>[2x]GPEFSMEDLIPLVNRLQDAFSAIGQNADLDLPQIAVVGGQSAGKSSVLENFVGRDFLPRGSGIVTRRPLVLQLVNATTEYAEFLHCKGKKFTDFEEVRLEIEAETDRVTGTNKGISPVPINLRVYSPHVLNLTLVDLPGMTKVPVGDQPPDIEFQIRDMLMQFVTKENCLILAVSPANSDLANSDALKVAKEVDPQGQRTIGVITKLDLMDEGTDARDVLENKLLP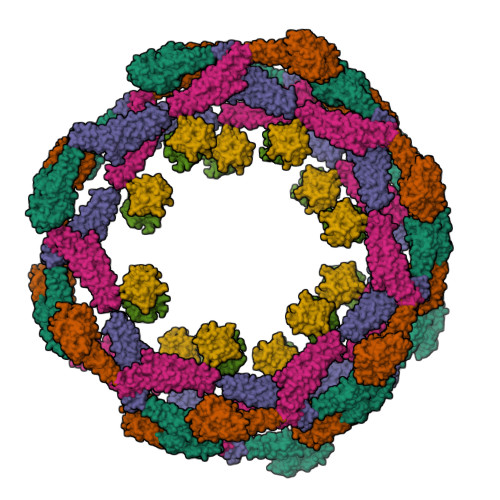LRRGYIGVVNRSQKDIDGKKDITAALAAERKFFLSHPSYRHLADRMGTPYLQKVLNQQLTNHIRDTLPGLRNKLQSQLLSIEKEVEEYKNFRPDKHGTDSRVDEMLRMYHALKEALSIIGNINTTTV;>[2x]MVVSEVDIAKADPAAASHPLLLNGDATVAQKNPGSVAENNLCSQYEEKVRPCIDLIDSLRALGVEQDLALPAIAVIGDQSSGKSSVLEALSGVALPRGSGIVTRCPLVLKLKKLVNEDKWRGKVSYQDYEIEISDASEVEKEINKAQNAIAGEGMGISHELITLEISSRDVPDLTLIDLPGITRVAVGNQPADIGYKIKTLIKKYIQRQETISLVVVPSNVDIATTEALSMAQEVDPEGDRTIGILTKPDLVDKGTEDKVVDVVRNLVFHLKKGYMIVKCRGQQEIQDQLSLSEALQREKIFFENHPYFRDLLEEGKATVPCLAEKLTSELITHICKSLPLLENQIKETHQRITEELQKYGVDIPEDENEKMFFLIDKVNAFNQDITALMQGEETVGEEDIRLFTRLRHEFHKWSTIIENNFQEGHKILSRKIQKFENQYRGRELPGFVNYRTFETIVKQQIKALEEPAVDMLHTVTDMVRLAFTDVSIKNFEEFFNLHRTAKSKIEDIRAEQEREGEKLIRLHFQMEQIVYCQDQVYRGALQKVREKELEEEKKKKSWDFGAFQSSSATDSSMEEIFQHLMAYHQEASKRISSHIPLIIQFFMLQTYGQQLQKAMLQLLQDKDTYSWLLKERSDTSDKRKFLKERLARLTQARRRLAQFPG;>[2x]ILVIRKGWLTINNIGIMKGGSKEYWFVLTAENLSWYKDDEEKEKKYMLSVDNLKLRDVEKGFMSSKHIFALFNTEQRNVYKDYRQLELACETQEEVDSWKASFLRAGVYPERV> MGFEFTLMVVGESGLGKSTLINSLFLTDLYPERVIPGAAEKIERTVQIEASTVEIEERGVKLRLTVVDTPGYGDAINCRDCFKTIISYI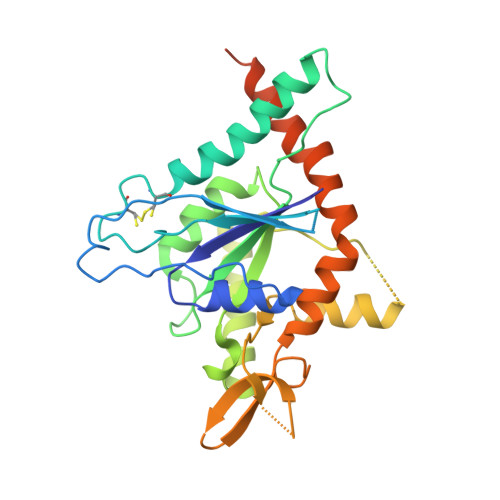DEQFERYLHDESGLNRRHIIDNRVHCCFYFISPFGHGLKPLDVAFMKAIHNKVNIVPVIAKADTLTLKERERLKKRILDEIEEHNIKIYHLPDAESDEDEDFKEQTRLLKASIPFSVVGSNQLIEAKGKKVRGRLYPWGVVEVENPEHNDFLKLRTMLITHMQDLQEVTQDLHYENFRSERLKRGGLESGKETAAAKFERNHMDSSTSAA>[3x]MDDISQDNFLLSKEYENSLDVDTKKASGIYYTPKIIVDYIVKKTLKNHDIIKNPYPRILDISCGCGNFLLEVYDILYDLFEENIYELKKKYDENYWTVDNIHRHILNYCIYGADIDEKAISILKDSLTNKKVVNDLDESDIKINLFCCDSLKKKWRYKFDYIVGNPPYIGHKKLEKKYKKFLLEKYSEVYKDKADLYFCF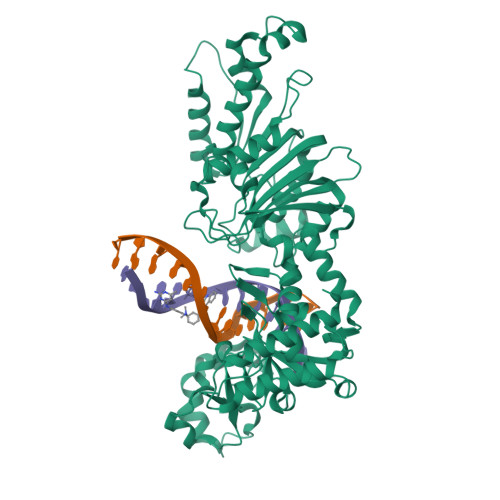YKKIIDILKQGGIGSVITPRYFLESLSGKDLREYIKSNVNVQEIVDFLGANIFKNIGVSSCILTFDKKKTKETYIDVFKIKNEDICINKFETLEELLKSSKFEHFNINQRLLSDEWILVNKDDETFYNKIQEKCKYSLEDIAISFQGIITGCDKAFILSKDDVKLNLVDDKFLKCWIKSKNINKYIVDKSEYRLIYSNDIDNENTNKRILDEIIGLYKTKLENRRECKSGIRKWYELQWGREKLFFERKKIMYPYKSNENRFAIDYDNNFSSADVYSFFIKEEYLDKFSYEYLVGILNSSVYDKYFKITAKKMSKNIYDYYPNKVMKIRIFRDNNYEEIENLSKQIISILLNKSIDKGKVEKLQIKMDNLIMDSLGI> MRKFNSHSIPIRLNLLFSIVILLFMTIIGRLLYMQVLNKDFYEKKLASASQTKVTTSSARGEIYDASGKPLVENTLKQVVSFTRSNKMTATDLKEIAKKLLTYVSISSPNLTERQLADYYLADPEIYKKTVEALPSEKRLDSDGNRLSESELYNNAVDSVPTSQLNYTEDEKKEIYLFSQLN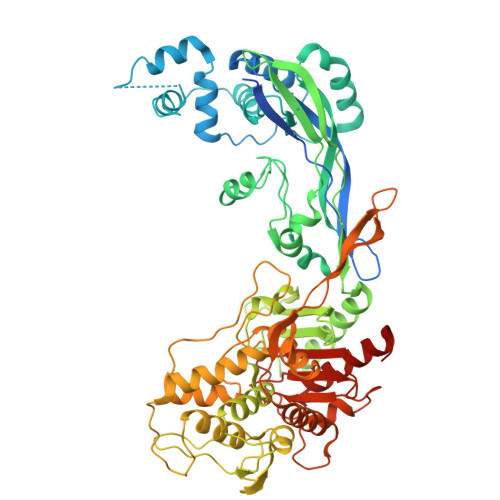AVGNFATGTIATDPLNDSQVAVIASISKEMPGISISTSWDRKILETSLSSIVGSVSSEKAGLPAEEAESYLKKGYSLNDRVGTSYLEKQYEEVLQGKRPVKEIHLDKHGDMESVENIEEGSKGKNIKLTIDLAFQDSVDALLKSYFNSELGNGGAKYSEGVYAVALNPQTGAVLSMSGLKHDLKTGELTPDSLGTVTNVFVPGSVVKAATISSGWENGVLSGNQTLTDQPIVFQGSAPIYSWYKLAYGSFPITAVEALEYSSNAYVVQTALGIMGQTYQPNMFVGTSNLESAMGKLRSTFGEYGLGSATGIDLPDESTGLVPKEYNFANFITNAFGQFDNYTPMQLAQYVATIANNGVRLAPHIVEGIYDNNDKGGLGELIQAIDTKEINKVNISESDMAILHQGFYQVSHGTSPLTTGRAFSDGATVSISGKTGTGESYVAGGQEANNTNAVAYAPTENPQIAVAVVFPHNTNLTKNVGPAIARDIINLYNQHHPMN1,4,7,10,13,16-HEXAOXACYCLOOCTADECANE | C12 H24 O6 | 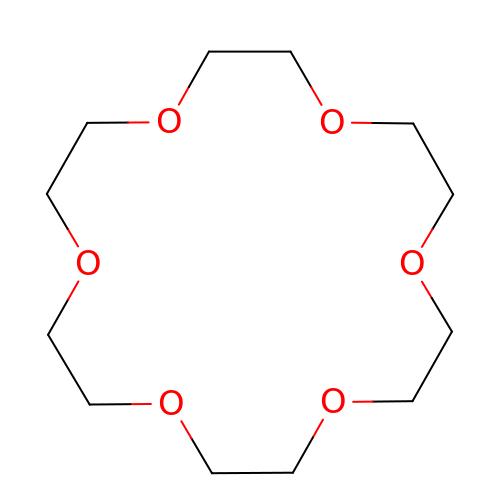XEZNGIUYQVAUSS-UHFFFAOYSA-N> DVSFRLSGADPSSYGMFIKDLRNALPHTEKVYNIPLLLPSVSGAGRYLLMHLFNYDGNTITVAVDVTNVYIMGYLALTTSYFFNEPAADLASQYVFRS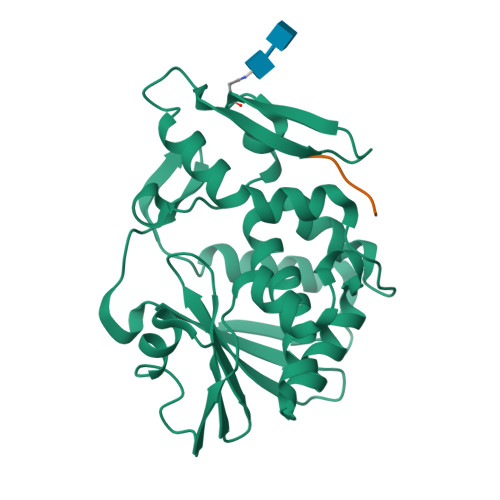ARRKITLPYSGNYERLQIAAGKPREKIPIGLPALDTAISTLLHYDSTAAAGALLVLIQTTAEAARFKYIEQQIQERAYRDEVPSSATISLENSWSGLSKQIQLAQGNNGVFRTPTVLVDSKGNRVQITNVTSNVVTSNIQLLLNTKNI;> SDDDMG>[2x]MIKQRTLKNIIRATGVGLHSGEKVYLTLKPAPVDTGIVFCRTDLDPVVEIPARAENVGETTMSTTLVKGDVKVDTVEHLLSAMAGLGIDNAYVELSASEVPIMDGSAGPFVFLIQSAGLQEQEAAKKFIRIKREVSVEEGDKRAVFVPFDGFKVSFEIDFDHPVFRGRTQQASVDFSSTSFVKEVSRARTFGFMRDIEYLRSQNLALGGSV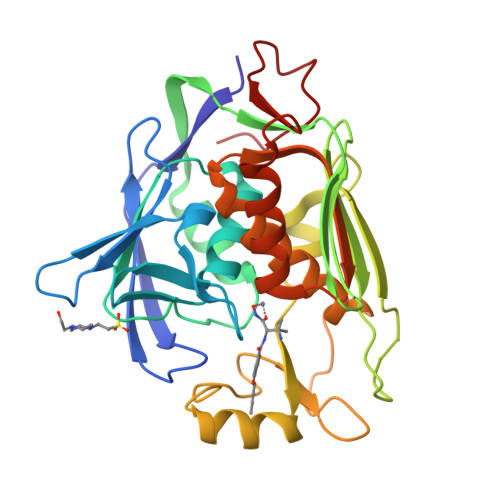ENAIVVDENRVLNEDGLRYEDEFVKHKILDAIGDLYLLGNSLIGEFRGFKSGHALNNQLLRTLIADKDAWEVVTFEDARTAPISYMRP> PIFLNVLEAIEPGVVCAGHDNNQPDSFAALLSSLNELGERQLVHVVKWAKALPGFRNLHVDDQMAVIQYSWMGLMVFAMGWRSFTNANSRMLYFAPDLVFNEYRMHKSRMYSQCVRMRHLSQEFGWLQITPQEFLCMKALLLFSIIPVDGLKNQKFFDELRMNYIKELDRIIACKRKNPTSCSRRFYQLTKLLDSVQPIARELHQFTFDLLIKSHMVSVDFPEMMAEIIS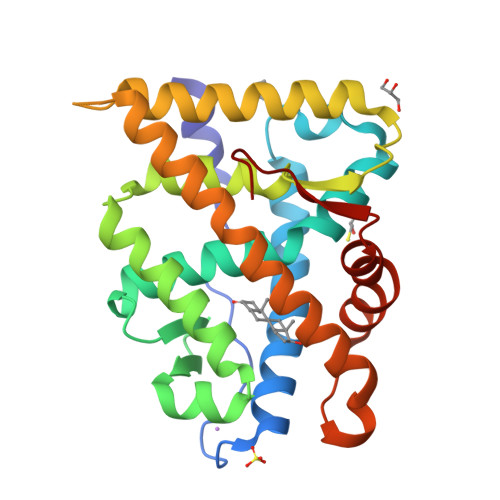VQVPKILSGKVKPIYFHTQ> TRINLTLVSE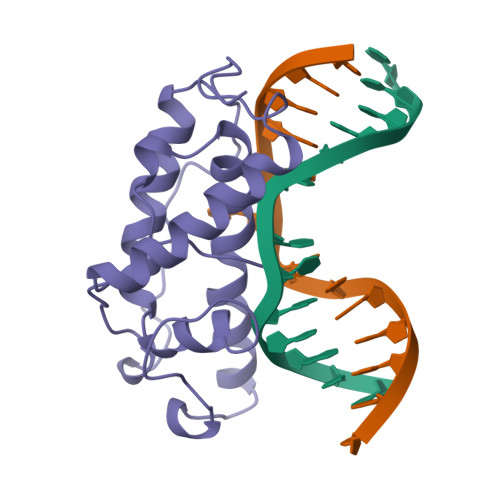LADQHLMAEYRQLPRVFGAVRKHVANGKRVRDFKISPTFILGAGHVTFFYDKLEFLRKRQIELIAECLKRGFNIKDTTVQDISDIPQEFRGDYIPHEASIAISQARLDEKIAQRPTWYKYYGKAIYA>YKKAGLQRTLVLIKPDAF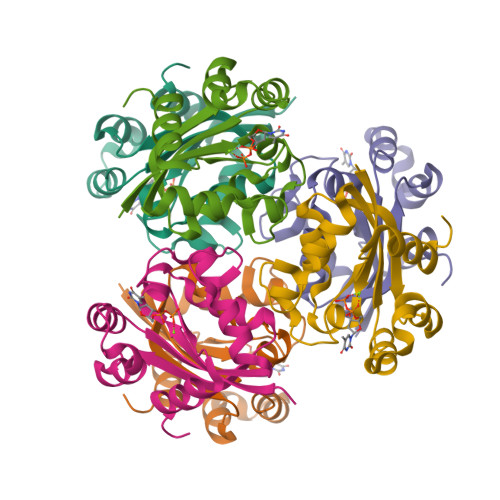ERSLVAEIMGRIEKKNFKIVSMKFWSKAPRNLIEQHYKEHSEQSYFNDNCDFMVSGPIISIVYEGTDAISKIRRLQGNILTPGTIRGDLANDIGENLIHASDSEDSAVDEISIWFPETKMETDN[6x]>[2x]DVAAMDFTDKLIISRPLYISDNADPKCGYCNGKKDSSHKFASPGWSDFYKGDEDKVELQSSTVGFNSELVNAETYDKLCNLGFRRSGSFMYKTDMLRNCCRLYTIRTNEKYLTMSKELKTSLKRFKKKITSPEFKPQPKYVSWIDELCDYEPKSTSFKAVFEPAEFTDEKYDLYVRYQHYIHSDEDNTPSQFESFLCDTPFTDSEITGTEKEWEQLNNWHNLQPGERVTKNGPAHECYYHNGKLIALSVLDFLPSGVSSVYFIWDPDYYDWSLGKVSALRELAL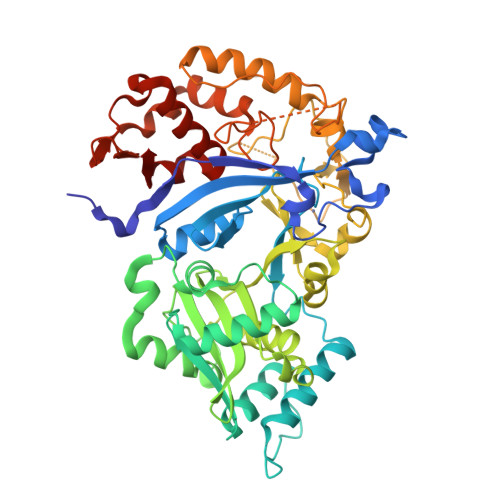VSKIGRPYYYLGYYIDDCPKMNYKAKFGGEILDVCNQKYVPLSKIHQIIKHNELFVGLNSTVASPDSEILITSASDKINFDEPFINAVDDIYGPNGNASQNAITSVAKLRKYGINYSPDLQRSIYKEIPNDGNSTSSASSDKKDVYRIPNVVPGLVPLMEIVSLFESGKMNELNNNVVLFDTKINALRIVRDFISEKPEIKTVITDVIRLIGLDNTKKAIIII> MSMDISDFYQTFFDEADELLADMEQHLLVLQPEAPDAEQLNAIFRAAHSIKGGAG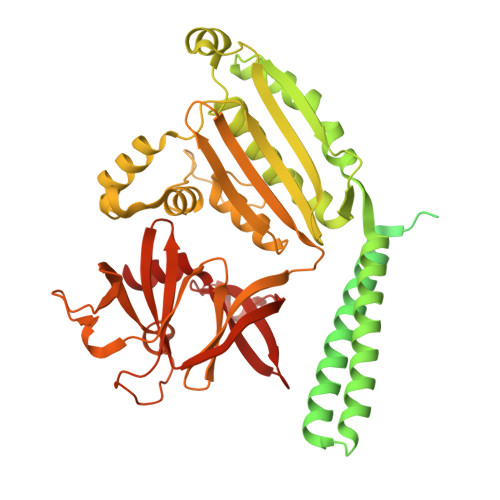TFGFSVLQETTHLMENLLDEARRGEMQLNTDIINLFLETKDIMQEQLDAYKQSQEPDAASFDYICQALRQLALEAKGETPSAVTRLSVVAKSEPQDEQSRSQSPRRIILSRLKAGEVDLLEEELGHLTTLTDVVKGADSLSAILPGDIAEDDITAVLCFVIEADQITFETVEVSPKISTPPVLKLAAEQAPTGRVEREKTTRSNESTSIRVAVEKVDQLINLVGELVITQSMLAQRSSELDPVNHGDLITSMGQLQRNARDLQESVMSIRMMPMEYVFSRYPRLVRDLAGKLGKQVELTLVGSSTELDKSLIERIIDPLTHLVRNSLDHGIELPEKRLAAGKNSVGNLILSAEHQGGNICIEVTDDGAGLNRERILAKAASQGLTVSENMSDDEVAMLIFAPGFSTAEQVTDVSGRGVGMDVVKRNIQKMGGHVEIQSKQGTGTTIRILLPLTLAILDGMSVRVADEVFILPLNAVMESLQPREADLHPLAGGERVLEVRGEYLPIVELWKVFNVAGAKTEATQGIVVILQSGGRRYALLVDQLIGQHQVVVKNLESNYRKVPGISAATILGDGSVALIVDVSALQAINREQRMANTAA> SHVDPRIQGELEKLNQSTDDINRRETELEDARQKFRSVLVEATVKLDELVKKIGKAVEDSKPY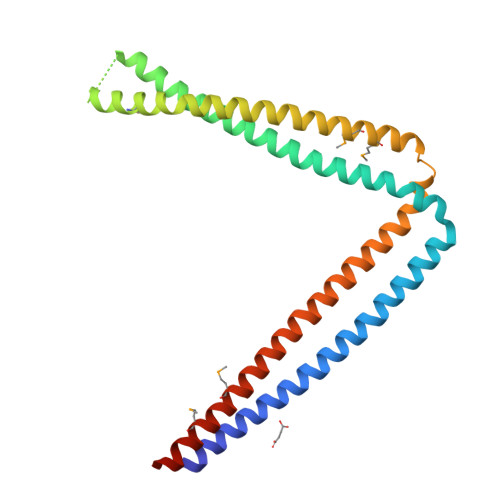WEARRVARQAQLEAQKATQDFQRATEVLRAAKETISLAEQRLLEDDKRQFDSAWQEMLNHATQRVAEAEQTKTRSELVHKETAARYNAAMGRMRQLEKKLKRAINKSKPYFELKAKYYVQLEQLKKTVDDLQAKLTLAKGEYKMALKNLEMISDEIHEAAASSAM>[2x]MDFKENPNLRDNWTDAEGYYRVNIGEVLDKRYNVYGYTGQGVFSNVVRARDNARANQEVAVKIIRNNELMQKTGLKELEFLKKLNDADPDDKFHCLRLFRHFYHKQHLCLVFEPLSMNLREVLKKYGKDVGLHIKAVRSYSQQLFLALKLLKRCNILHADIKPDNILVNESKTILKLCDFGSASHVADNDITPYLVSRFYRAPEIIIGKSYDYGIDMWSVGCTLYELYTGKILF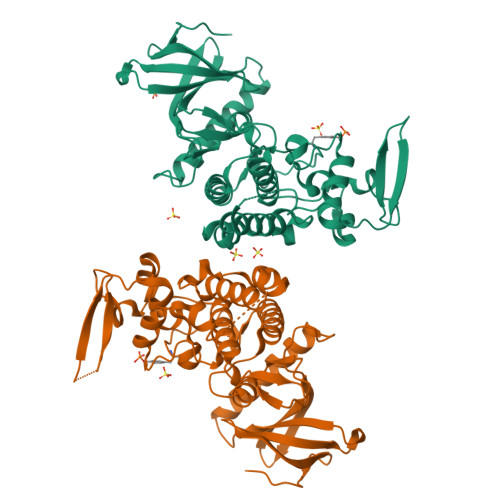PGKTNNHMLKLAMDLKGKMPNKMIRKGVFKDQHFDQNLNFMYIEVDKVTEREKVTVMSTINPTKDLLADLIGCQRLPEDQRKKVHQLKDLLDQILMLDPAKRISINQALQHAFIQEKIHHHHHH>[4x]AKEIPIGKPQLLGGMEIAAVYL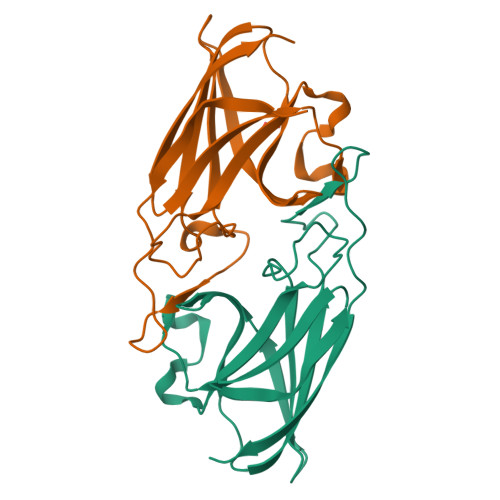QPIEMEPEGMMRPAKDSDVHLEADIKAAKDNTNGFAEGDWVPYLVVSYELTHLDNGKVQKGDFMPMVANDGPHYGDNVKLDGPGKYKLKLFVSPPSANQHAHFGRAVDKETGVGPWFKPVTAEYEFVYAGTGKKGAY> GSPLPWCPHLVAVCPIPAAGLDVTQPCGDCGTIQENWVCLSCYQVYCGRYINGHMLQHHGNSGHPLVLSYIDLSAWCYYCQAYVHHQALLDVKNIAHQNKFGEDMPH

HDAC6 is a structurally distinct microtubule-associated cytosolic deacetylase, harboring two tandem catalytic deacetylase domains2,3 and a zinc-finger ubiquitin-binding domain (UBD).4−6 The catalytic domains interact with dynein to transport aggregated proteins via microtubules to the aggresome for degradation,7−9 whereas the UBD binds free C-terminal diglycine motifs of polyubiquitin or polyISG chains associated with protein aggregates or other cargo. We previously identified and characterized the first small molecule binders of HDAC6-UBD, which can displace the native C-terminal ubiquitin RLRGG peptide from a narrow and deep pocket within this domain. These compounds have a carboxylate that mimics the C-terminus of the ubiquitin substrate and an extended aromatic structure that forms π-stacking interactions with W1182 and R1155.

The co-crystal structure also reveals that the N-Methyl group of 1 could be extended into the adjacent pocket to make additional interactions with the residues lining this site. To test this hypothesis, we first explored simple N-alkyl groups such as cyclopropylmethyl and benzyl groups, which could potentially extend into the side pocket, but they led to a significant loss of activity (data not shown). Therefore, we explored extended linker groups, starting from the corresponding methylacetamide derivative, which was synthesized according to Scheme 1. Compared to 1, the corresponding methylacetamide derivative showed a ∼4-fold loss of binding activity. In the co-crystal structure, R1155 moves to open the side pocket. The carbonyl and NH groups of the amide of 9 make additional hydrogen bonds with R1155 and Y1189, respectively, compared to 1, while maintaining the π-stacking of the quinazolinone core with R1155 and W1182 and hydrogen bond of the carboxylate with G1154 and Y1184. The co-crystal structure with 9 indicated that other larger amide groups could be extended into the side pocket to further improve activity.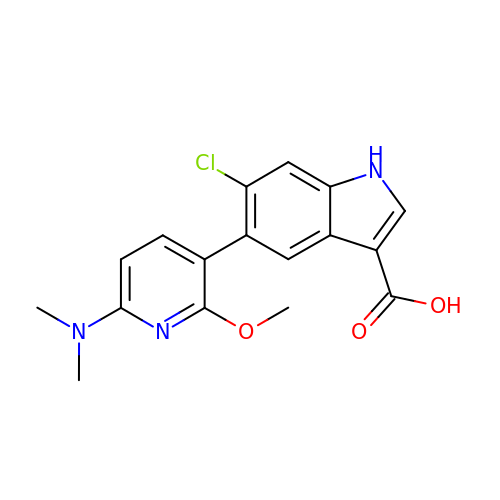6-chloro-5-[6-(dimethylamino)-2-methoxypyridin-3-yl]-1H-indole-3-carboxylic acid | C17 H16 Cl N3 O3 | MJHBRTGGZYSCHJ-UHFFFAOYSA-N>MTKPVLQDGETVVSQGTHAAIASELQAIAPEVAQSLAEFFAVLADPNRLRLLSLLARSELSVGDLAQAIGVSESAVSHQLRSLRNLRLVSYRKQGRHVYYQLQDHHIVAL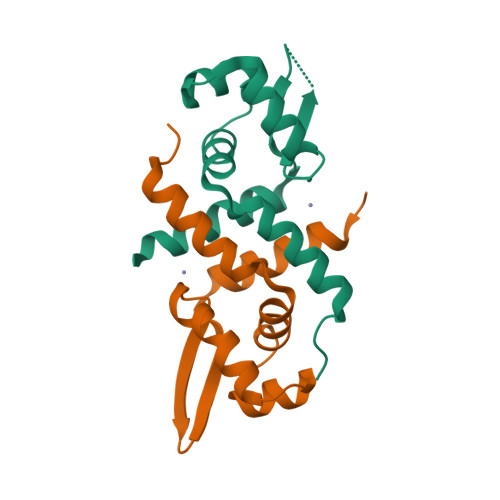YQNALDHLQESR[2x]>[4x]SNAMVDTFVKHKVKDISLAAWGRKEIELAEAEMP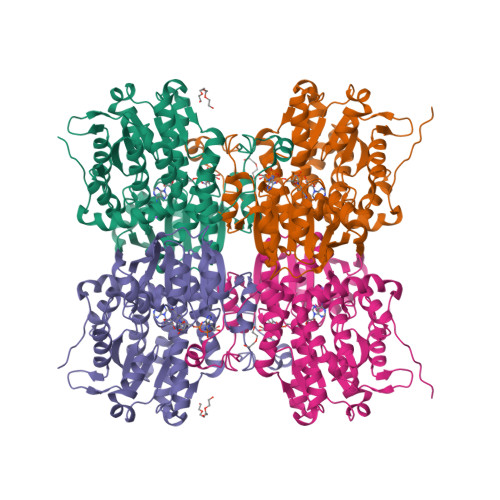GLMSIRKEFGPSKPLKGARVAGCLHMTIQTAVLIETLIELGAEVTWSSCNIFSTQDHAAAAIAAAGISVYAWKGMNEEEFDWCIEQTLFFGEDRKPLNMILDDGGDLTNMVLDRFPELVKDIRGISEETTTGVLRLKDRERNGSLVLPAININDSVTKSKFDNKYGCKESLVDSIRRATDVMMAGKVAVVAGYGDVGKGSAASLRGAGARVIVTEIDPICALQAAMDGYEVKKMADAVKRADIVVTATGNKNIITGEHFKAMRDKVIVCNIGHFDNEIDMAWLNKTYGSTKVTVKPQVDIYNVDGHDVIILAEGRLVNLGCATGHPSFVMSSSFSNQVIAQLELWENSSKYENKVYTLPKSLDEKVARLHLSKIDVELDILSADQAAYIGVTVDGPYKNDEYRY> KTSDANETEDHLESLICKVGEKSACSLESNLEGLAGVLEADLPNYKSKILRLLCTVARLLPEKLTIYTTLVGLLNARNYNFGGEFVEAMIRQLKESLKANNYNEAVYLVRFLSDLVNCHVIAAPSMVAMFENFVSVTQEEDVPQVRRDWYVYAFLSSLPWVGKELYEKKDAEMDRIFANTESYLKRRQKTHVPMLQVWTADKPHPQEEYLDCLWAQIQKLKKDRWQERHILRPYLAFDSILCEALQHNLPPFTPPPHTEDSVYPMPRVIFRMFDYTDDPEGPVMPGSHSVERFVIEENLHCIIKSHWKERKTCAAQLVSYPGKNKIPLNYHIVEVIFAELFQLPAPPHIDVMYTTLLIELCKLQP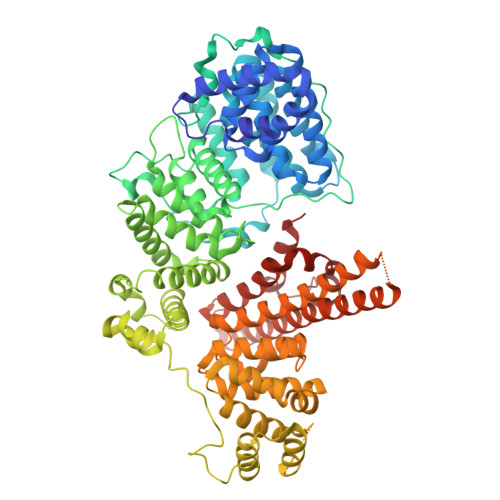GSLPQVLAQATEMLYMRLDTMNTTCVDRFINWFSHHLSNFQFRWSWEDWSDCLSQDPESPKPKFVREVLEKCMRLSYHQRILDIVPPTFSALCPSNPTCIYKYGDESSNSLPGHSVALCLAVAFKSKATNDEIFSILKDVPNPNQDDDDDEGFSFNPLKIEVFVQTLLHLAAKSFSHSFSALAKFHEVFKTLAESDEGKLHVLRVMFEVWRNHPQMIAVLVDKMIRTQIVDCAAVANWIFSSELSRDFTRLFVWEILHSTIRKMNKHVLKIQKELEEAKEKLARQHKRRSDDDDRSSDRKDGVLEEQIERLQEKVESAQSEQKNLFLVIFQRFIMILTEHLVRCETDGTSVLTPWYKNCIERLQQIFLQHHQIIQQYMVTLENLLFTAELDPHILAVFQQFCALQA> GAGCAGACCAGA;> CGGGACTCA;> TCTCCG;> TCTGAG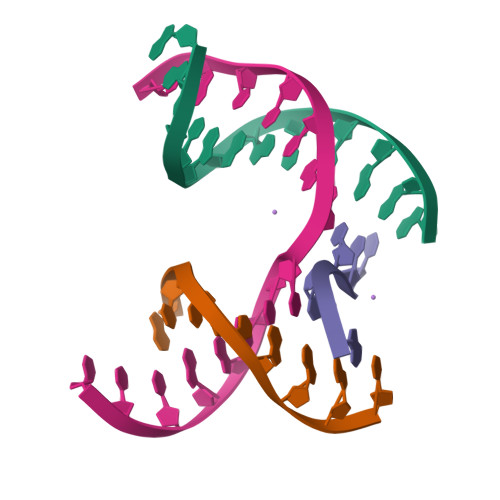TCGGTCTGC1-(4-fluorophenyl)-~{N}-[[(2~{R})-oxolan-2-yl]methyl]methanamine | C12 H16 F N O | 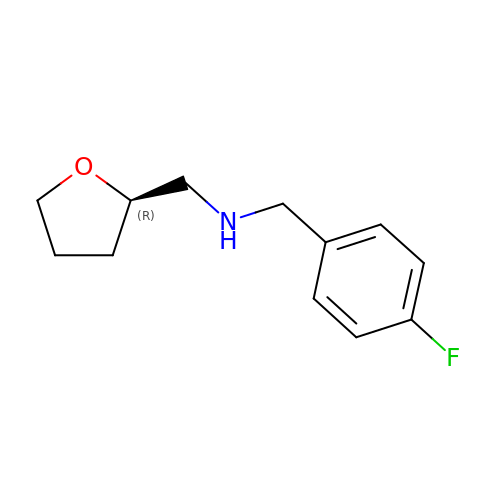SLYWRVMUMWKSOX-GFCCVEGCSA-N> MSIAVTGATGQLGGLVIQHLLKKVPAS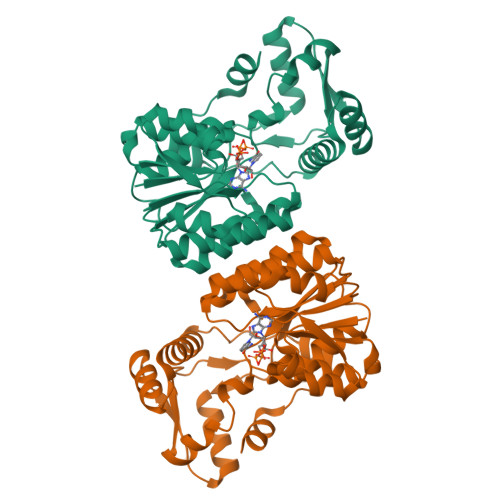QIIAIVRNVEKASTLADQGVEVRHGDYNQPESLQKAFAGVSKLLFISGPHYDNTLLIVQHANVVKAARDAGVKHIAYTGYAFAEESIIPLAHVHLATEYAIRTTNIPYTFLRNALYTDFFVNEGLRASTESGAIVTNAGSGIVNSVTRNELALAAATVLTEEGHENKTYNLVSNQPWTFDELAQILSEVSGKKVVHQPVSFEEEKNFLVNAGVPEPFAEITAAIYDAISKGEASKTSDDLQKLIGSLTPLKETVKQALKM> GHME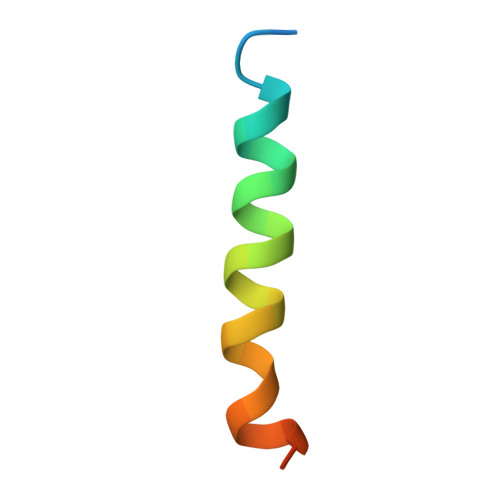DRLERLQEILRKFLYLEREFRQITIS>[2x]MSDLGSEELEEEGENDLGEYEGERNEVGERHGHGKARLPNGDTYEGSYEFGKRHGQGTYKFKNGARYTGDYVKNKKHGQGTFIYPDGSRYEGEWADDQRHGQGVYYYVNNDTYTGEWFNHQRHGQGTYLYAETGSKYVGTWVHGQQEGAAELIHLNHRYQGKFMNKNPVGPGKYVFDIGCEQHGEYRLTDTERGEEEEEEETLVNIVPKWKALNITELALWTPTLSEEQPPPEGQGQEEPQGLTGVGDPSEDIQAEGFEGELEPRGADEDVDTFRQESQENSYDIDQGNLNFDEEPSDLQD;>[2x]MENSTSLKQEKENQEPGEAERLWQGESDVSPQEPGPPSPEYREEEQRTDTEPAPRMSPSWSHQSRVSLSTGDLTAGPEVSSSPPPPPLQFHSTPLNTETTQDPVAASPTEKTANGIADTGTPYSDPWESSSAAKQSTSHYTSHAEESTFPQSQTPQPDLCGLRDASRNKSKHKGLRFDLLQEEGSDSNCDPDQPEVGASEAAQSMLEVAIQNAKAYLLSTSSKSGLNLYDHLSKVLTKILDERPADAVDIIENISQDVKMAHFNKKLDTLHNEYEMLPAYEIAETQKALFLQGHLEGADSELEEEMAESSLPNVMESAYYFEQAGVGLGTDETYRVFLALKQLTDTHPIQRCRFWGKILGLEMNYIVAEVEFRDGEDEEEVEEEGIAEERDNGGSEAGEEEEEELPKSLYKAPQVIPKEESRTGANKYVYFVCNVPGRPWVRLPSVTPAQIVTARKIKKFFTGRLDAAVISYPPFPGNESNYLRAQIARISAGTHVSPLGFYQFGEEEGEEEEVEGGRDSYEENPDFEGIQVIDLVESLSNWVHHVQYILPQGRCNWFNPIQKDEDEEEEEEEDEEKGEEPDYIEQEVGPPLLTPISEDLGIQNIPSWTTQLSSNLIPQYAIAVLRS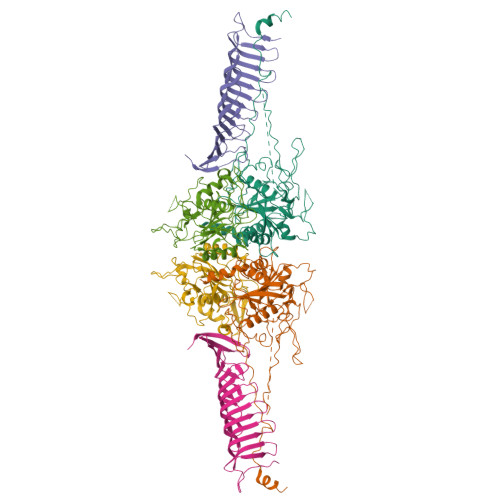NLWPGAYAFSNGKKFENFYIGWGHKYCVENYTPPSPPPVYQEYPSGPEITEMNDPSVEEEQAFRMTQEPVALSTEENEGTEDEDEDDED;>[2x]MDADSLLLSLELASGSGQGLSPDRRASLLTSLMLVKRDYRFARVLFWGRILGLVADYYIAQGLSEDQLAPRKTLYSLNCTEWSLLPPATEEMAMQISVVSGRFMGDPSHEYEHTELQKVNEGEKVFDEEVVVQIKEETRLVSIIDQIDKAVAIIPRGALFKTPFGVTHVNRTFEGLPLSEVRKLSSYFHFREAIDLKNKTLLEKSDLEPSLDFLDSLEYDIPRGSWSIQMERGNALVVLRSLLWPGLTFYHAPRTKNYGYIYVGTGEKNMDLPFML> MNLTIPFAKGHATENDFIIIPDEDARLDLTPEMVVTLCDRRAGIGADGILRVVKAADVEGSTVDPSLWFMDYRNADGSLAEMCGNGVRLFAHWLYSRGLVDNT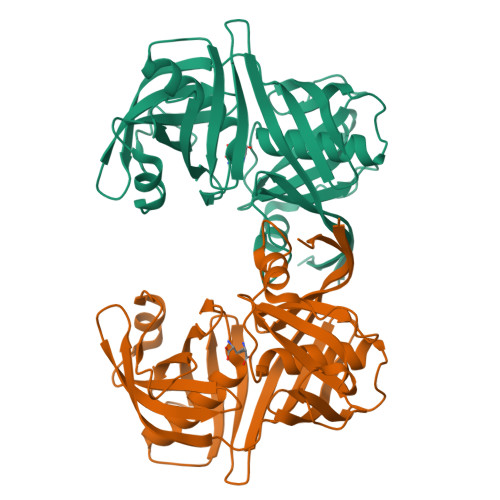SFDIGTRAGVRHVDILQADQHSAQVRVDMGIPDVTGLSTCDINGQVFAGLGVDMGNPHLACVVPGLSASALADMELRAPTFDQEFFPHGVNVEIVTELEDDAVSMRVWERGVGETRSCGTGTVAAACAALADAGLGEGTVKVCVPGGEVEVQIFDDGSTLTGPSAIIALGEVQIHHHHHH> GPLGSWSWESYLEEQKAITAPVSLFQDSQAVTHNKNGFKLGMKLEGIDPQHPSMYFILTVAEVCGYRLRLHFDGYSECHDFWVNANSPDIHPAGWFEKTGHKLQPPKGYKEEEFSWSQYLRSTRAQAAPKHLFVSQSHSPPPLGFQVGMKLEAVDRMQPSLVCVASVTDVVDSRFLVHFDNWDDTYDYWCDPSSPYIHPVGWCQKQGKPLTPPQDYPDP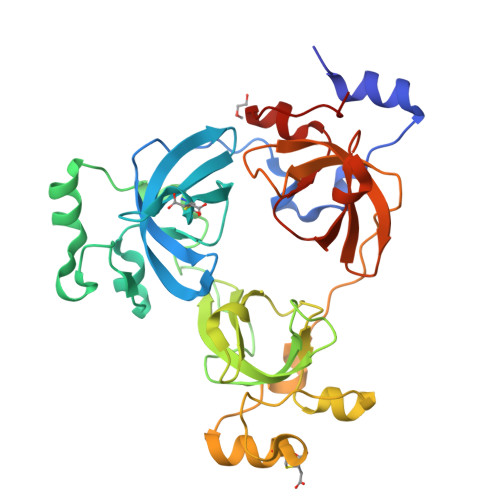DNFCWEKYLEETGASAVPTWAFKVRPPHSFLVNMKLEAVDRRNPALIRVASVEDVEDHRIKIHFDGWSHGYDFWIDADHPDIHPAGWCSKTGHPLQPPLG>SNAMLQLQNISVDYATPHVVKISLNRERQANSLSLALLEELQNILTQINEEANTRVVILTGAGEKAFCAGADLKERAGMNEEQVRHAVSMIRTTMEMVEQLPQPVIAAINGIALGGGTELSLACDFRIAAESASLGLTETTLAIIPGAGGTQRLPRLIGVGRAKELIYTGRRISAQEAKEYGLVEFV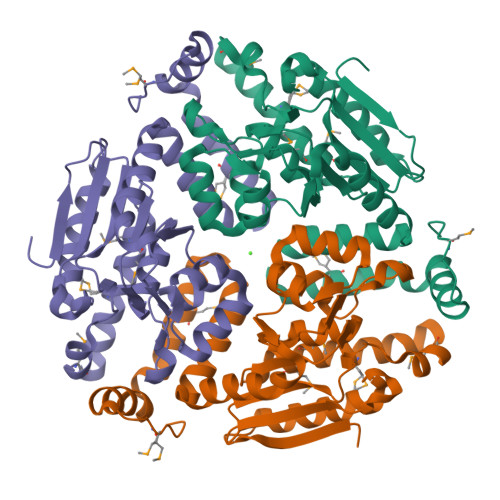VPVHLLEEKAIEIAEKIASNGPIAVRLAKEAISNGIQVDLHTGLQMEKQAYEGVIHTKDRLEGLQAFKEKRTPMYKGE[6x]>[4x]IQIN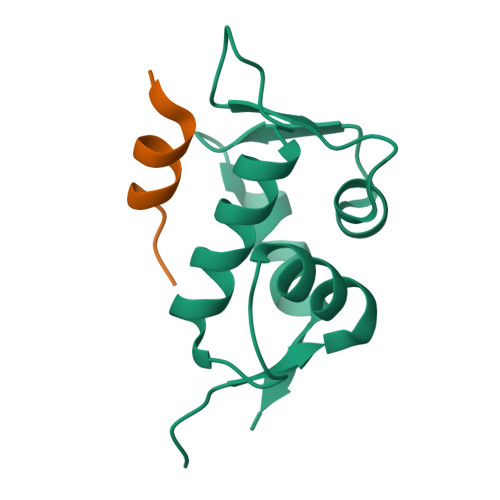QVRPKLPLLKILHAAGAQGEMFTVKEVMHYLGQYIMVKQLYDQQEQHMVYCGGDLLGELLGRQSFSVKDPSPLYDMLRKNLVTLAT;>SQETFSDLWKLLPEN[4x]>MEERTLVILGATGSIGTQTLDVLKKVKGIRLIGISFHSNLELAFKIVKEFNVKNVAITGDVEFEDSSINVWKGSHSIEEMLEALKPDITMVAVSGFSGLRAVLASLEHSKRVCLANK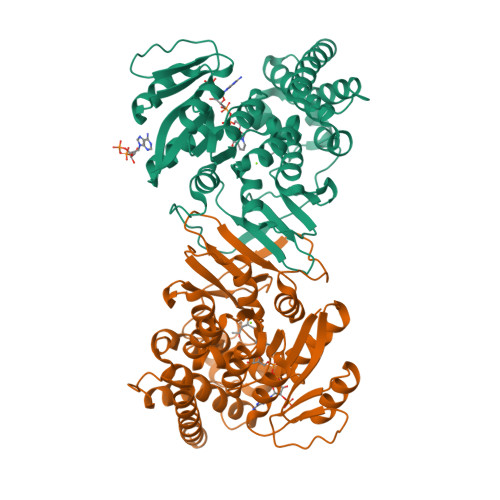ESLVCGGFLVKKKLKEKGTELIPVDSEHSAIFQVMEPEVEKVVLTASGGALRDWKISKIDRARPEDVLKHPVWNMGARITVDSATMVNKAFEVLEAMELFELPFEKIEVKIHREGLVHGAVVLPDGNVKMVVSPPDMRIPISYALFYPRRVALEPFFLRTISLSFEDPDPEKYPAFFLLKEIKDSYALRTAFNAADEVAVEAFLKGRIRFGGIHRVIEKTLEEFQGYPQPRTLDDVERIHFEAIKKAERVTEWLSSTSY[2x]> MKESYYSIGEVSKLANVSIKALRYYDKIDLFKPAYVDPDTSYRYYTDSQLIHLDLIKSLKYIGTPLEEMKKAQDLEMEELFAFYTEQERQIREKLDFLSALEQTISLVKKRMKRQMEYPALGEVFVLDEEEIRIIQTEAEGLG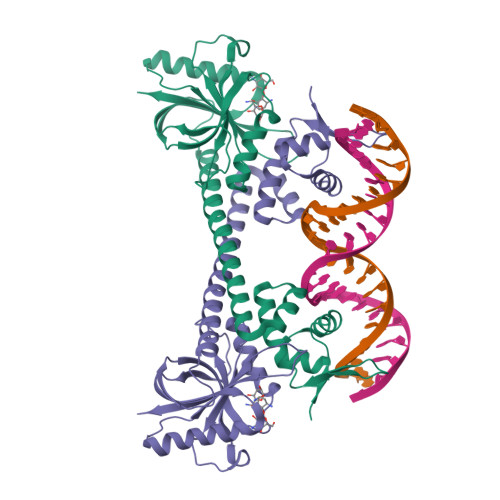PENVLNASYSKLKKFIESADGFTNNSYGATFSFQPYTSIDEMTYRHIFTPVLTNKQISSITPDMEITTIPKGRYACIAYNFSPEHYFLNLQKLIKYIADRQLTVVSDVYELIIPIHYSPKKQEEYRVEMKIRILDHHHHHH Transcription activator-like (TAL) effectors specifically bind to double stranded (ds) DNA through a central domain of tandem repeats. Each TAL effector (TALE) repeat comprises 33–35 amino acids and recognizes one specific DNA base through a highly variable residue at a fixed position in the repeat. The crystal structures of TAL effector (TALE) proteins bound to their respective target DNAs have revealed that the residue at position 13 is the only one directly involved in DNA base recognition, whereas the 12th residue stabilizes the proper loop conformation. dHax3, an engineered TALE protein, proved to be a useful scaffold for structural characterizations. We then present fifteen crystal structures of engineered dHax3 variants in complex with target DNA molecules, which elucidate the structural basis for the recognition of bases adenine (A) and guanine (G) by reported or uncharacterized TALE codes.

When the natural TALE codes were discovered, no code was found highly specific for base G. In light of the structures of the DNA-binding zinc finger proteins where positive charged amino acids such as Arg, His, Lys play a critical role in the coordination of base G, we made a dHax3 variant with an Arg34, His34, Lys34 in the 7th repeat. We then attempted to co-crystallize these proteins with a modified dHax3 box element whose 7th base is changed from A to G. Four complex structures were determined at high resolutions. Nevertheless, an independent study showed that Gln34 is highly specific for base G, but not for base A. Therefore, Gln34 may be a good code that can discriminate G from A. It was shown that His34 is a strong code for base G, but not for base A. The structures shown here provide the molecular basis for the distinctive recognition of G and A by His34. Notably, the newly determined structures reported in this manuscript show that His34 forms H-bond with base G, but not with base A, which consolidates the genetic observation that His34 is a strong and specific code for base G. The structures also suggest that Gln34 and Asn34 are both strong codes for base G. Gln34, highly specific for base G, was not reported before and should be further exploited. Nevertheless, the discriminative binding of A and G by Asn34 or His34 unveiled by the structures provide unprecedented clarity to understand the biochemical observations. His34/Gln34 → G and Asp34 → C can be used as strong codes.

>[2x]MQWSGARALEALLTVAGELRGPPLQLDTGQLLKIAKRGGVTAVEAVHAWRNALTGAPLNLTPEQVVAIASHDGGKQALETVQRLLPVLCQAHGLTPQQVVAIASHDGGKQALETVQRLLPVLCQAHGLTPEQVVAIASHDGGKQALETVQALLPVLCQAHGLTPEQVVAIASNGGGKQALETVQRLLPVLCQAHGLTPQQVVAIASNGGGKQALETVQRLLPVLCQAHGLTPQQVVAIASNGGGKQALETVQRLLPVLCQAHGLTPQQVVAIASNHGGKQALETVQRLLPVLCQAHGLTPQQVVAIASNGGGKQALETVQRLLPVLCQAHGLTPQQVVAIASHDGGKQALETVQRLLPVLCQAHGLTPEQVVAIASNGGGKQALETVQRLLPVLCQAHGLTPEQVVAIASHDGGKQALETVQRLLPVLCQAHGLTPQQVVAIASNGGGRPALESIVAQLSRPDPALAALTNDHLVALACLGGRPALDAVKKLEHHHHHH>[2x]METDNVELAQSKRKVVLAEQGSFYIGGRTVTGPGKFDPSKPVIRYSNEGATFYINQMYVNFQAPVRPRGLPLVFWHGGGLTGHIWESTPDGRPGFQTLFVQDRHTVYTIDQPGRGRGNIPTFNGPFGQLEEESIVNTVTGNSSKEGAWVRDRLGPAPGQFFENSQFPRGYEDNYFKEMGFSPSISSDEIVDAVVKLVTHIGPCVLVTHSASGVLGMRVATHAKNVRGIVAYEPATSIFPKGKVPEIPPL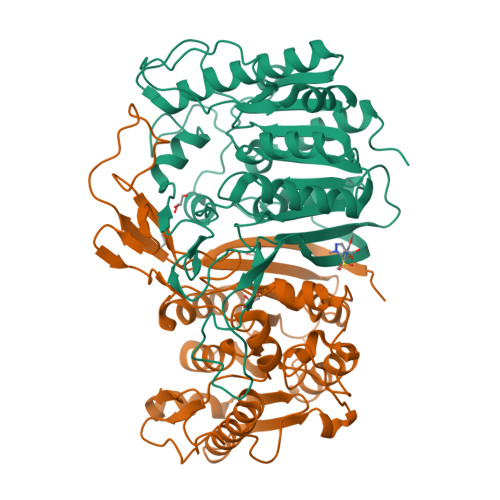ADKKSQIFPPFEIQESYFKKLAKIPIQFVFGDNIPKNPKSAYWFLDWWRVTRYAHSLSLEAINKLGGQASLLDLPTAGLRGNTHFPFTDRNNVQVASLLSDFLGKHGLDQNESLEHHHHHH> MGSDKIHHHHHHENLYFQGMQVIKQKLTATCAQLTGYLHQPDTNAHQTNLPAIIIVPG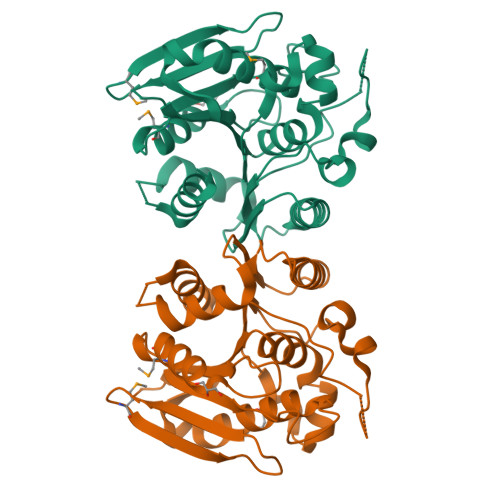GSYTHIPVAQAESLAMAFAGHGYQAFYLEYTLLTDQQPLGLAPVLDLGRAVNLLRQHAAEWHIDPQQITPAGFSVGGHIVALYNDYWATRVATELNVTPAMLKPNNVVLGYPVISPLLGFPKDDATLATWTPTPNELAADQHVNSDNQPTFIWTTADDPIVPATNTLAYATALATAKIPYELHVFKHGPHGLALANAQTAWKPDANQPHVAHWLTLALEWLADNR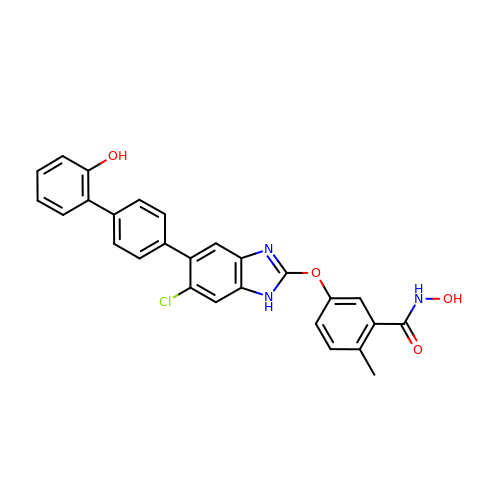5-{[6-chloro-5-(2'-hydroxy[1,1'-biphenyl]-4-yl)-1H-benzimidazol-2-yl]oxy}-N-hydroxy-2-methylbenzamide | C27 H20 Cl N3 O4 | YSNIPFQCRHRGSO-UHFFFAOYSA-N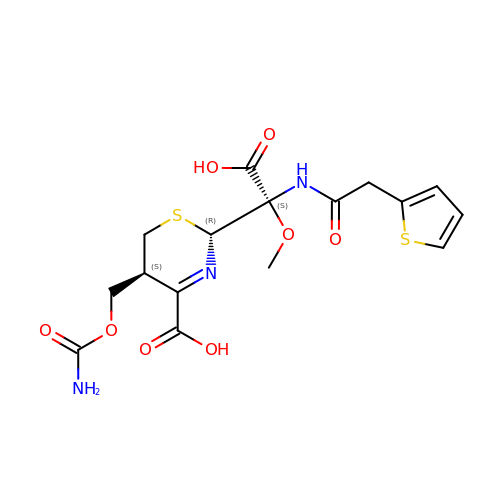(2~{R},5~{S})-5-(aminocarbonyloxymethyl)-2-[(1~{S})-1-methoxy-2-oxidanyl-2-oxidanylidene-1-(2-thiophen-2-ylethanoylamino)ethyl]-5,6-dihydro-2~{H}-1,3-thiazine-4-carboxylic acid | C16 H19 N3 O8 S2 | GMTLEACBDXZSEB-SGEDMPRTSA-N>MSEFNITETYLRFLEEDTEMTMPIAAIEALVTLLRIKTPETAAEMINTIKSSTEELIKSIPNSVSLRAGCDIFMRFVLRNLHLYGDWENCKQHLIENGQLFVSRAKKSRNKIAEIGVDFIADDDIILVHGYSRAVFSLLNHAANKFIRFRCVVTESRPSKQGNQLYTLLEQKGIPVTLIVDSAVGAVIDKVDKVFVGAEGVAESGGIINLVGTYSVGVLAHNARKPFYVVTESHKFVRMFPLSSDDLPMAGPPLDFTRRTDDLEDALRGPTIDYTAQEYITALITDLGVLTPSAVSEELIKMWYD[2x];>MSESEAKSRSATPPSKAKQATPTTTAAANGEKKLTNKELKELKKQEKAAKRAAMKQANGISIEQQQQQAQMKKEKKQLQREQQQKREQKQKNANKKKQNERNVKKSTLFGHLETTEERRATILALTSAVSSPKTSRITAAGLMVPVVASALSGSNVLTASSLMPVGPNASSTVSASAPASTTTTLPASSAALSAGTSSASTNTPTAIQQEIASSNASDVAKTLASISLEAGEFNVIPGISSVIPTVLEQSFDNSSLISSVKELLLNKDLIHPSILLLTSHLAHYKIVGSIPRCIAMLEVFQIVIKDYQTPKGTTLSRNLTSYLSHQIDLLKKARPLSVTMGNAIRWLKQEISLIDPSTPDKAAKKDLCEKIGQFAKEKIELADQLIIDNASTQIEESTTIVTYGSSKVLTELLLHNAISLKKNIKVIVVDSRPLFEGRKMAETLRNAGVNVMYALITSLDTIFNMDVDYVFLGAHSILSNGFLYSRAGTAMLAMSAKRRNIPVLVCCESLKFSQRVQLDSVTFNELADPNDLVNIDYENPVERRGNKGALLNQFIKERKFEKKKLAMENKPKGNKIGGKKGSEGESKDASNEEDSNSKNILDGWQELPSLNIVNILYDLTPPEYIKKVITEFGALPPSSVPVILREYKGSA[2x];>[2x]MSSQAFTSVHPNAATSDVNVTIDTFVAKLKRRQVQGSYAIALETLQLLMRFISAARWNHVNDLIEQIRDLGNSLEKAHPTAFSCGNVIRRILAVLRDEVEEDTMSTTVTSTSVAEPLISSMFNLLQKPEQPHQNRKNSSGSSSMKTKTDYRQVAIQGIKDLIDEIKNIDEGIQQIAIDLIHDHEILLTPTPDSKTVLKFLITARERSNRTFTVLVTEGFPNNTKNAHEFAKKLAQHNIETLVVPDSAVFALMSRVGKVIIGTKAVFVNGGTISSNSGVSSVCECAREFRTPVFAVAGLYKLSPLYPFDVEKFVEFGGSQRILPRMDPRKRLDTVNQITDYVPPENIDIYITNVGGFNPSFIYRIAWDNYKQIDVHLDKNKA;>MAGKKGQKKSGLGNHGKNSDMDVEDRLQAVVLTDSYETRFMPLTAVKPRCLLPLANVPLIEYTLEFLAKAGVHEVFLICSSHANQINDYIENSKWNLPWSPFKITTIMSPEARCTGDVMRDLDNRGIITGDFILVSGDVLTNIDFSKMLEFHKKMHLQDKDHISTMCLSKASTYPKTRTIEPAAFVLDKSTSRCIYYQDLPLPSSREKTSIQIDPELLDNVDEFVIRNDLIDCRIDICTSHVPLIFQENFDYQSLRTDFVKGVISSDILGKHIYAYLTDEYAVRVESWQTYDTISQDFLGRWCYPLVLDSNIQDDQTYSYESRHIYKEKDVVLAQSCKIGKCTAIGSGTKIGEGTKIENSVIGRNCQIGENIRIKNSFIWDDCIIGNNSIIDHSLIASNATLGSNVRLNDGCIIGFNVKIDDNMDLDRNTKISASPLKNAGSRMYDNESNEQFDQDLDDQTLAVSIVGDKGVGYIYESEVSDDEDSSTEACKEINTLSNQLDELYLSDDSISSATKKTKKRRTMSVNSIYTDREEIDSEFEDEDFEKEGIATVERAMENNHDLDTALLELNTLRMSMNVTYHEVRIATITALLRRVYHFIATQTLGPKDAVVKVFNQWGLLFKRQAFDEEEYIDLMNIIMEKIVEQSFDKPDLILFSALVSLYDNDIIEEDVIYKWWDNVSTDPRYDEVKKLTVKWVEWLQNADEESSSEEE[2x];>[2x]MSIQAFVFCGKGSNLAPFTQPDFPFQTQNKDSTAATSGDKLNELVNSALDSTVINEFMQHSTRLPKALLPIGNRPMIEYVLDWCDQADFKEISVVAPVDEIELIESGLTSFLSLRKQQFELIYKALSNSNHSHHLQDPKKINFIPSKANSTGESLQKELLPRINGDFVILPCDFVTDIPPQVLVDQFRNRDDNNLAMTIYYKNSLDSSIDKKQQQKQKQQQFFTVYSENEDSERQPILLDVYSQRDVTKTKYLQIRSHLLWNYPNLTVSTKLLNSFIYFCSFELCQLLKLGPQSMSRQASFKDPFTGNQQQQNPPTTDDDEDRNHDDDDDYKPSATSIQPTYFKKKNDLILDPINCNKSLSKVFRDLSRRSWQHSKPREPIGIFILPNETLFIRANNLNAYMDANRFVLKIKSQTMFTKNIQIQSAAIGADAIVDPKCQISAHSNVKMSVLGTQANIGSRCRVAGSLLFPGVHLGDEVILENCIIGPMAKIGSKCKLSNCYIEGHYVVEPKNNFKGETLANVYLDEDEEDELIYDDSVIAGESEIAEETDSDDRSDEDSDDSEYTDEYEYEDDGLFER;>MSTSHCRFYENKYPEIDDIVMVNVQQIAEMGAYVKLLEYDNIEGMILLSELSRRRIRSIQKLIRVGKNDVAVVLRVDKEKGYIDLSKRRVSSEDIIKCEEKYQKSKTVHSILRYCAEKFQIPLEELYKTIAWPLSRKFGHAYEAFKLSIIDETVWEGIEPPSKDVLDELKNYISKRLTPQAVKIRADVEVSCFSYEGIDAIKDALKSAEDMSTEQMQVKVKLVAAPLYVLTTQALDKQKGIEQLESAIEKITEVITKYGGVCNITMPPKAVTATEDAELQALLESKELDNRSDSEDDEDESDDE[2x];>[2x]MSSDLAAELGFDPALKKKKKTKKVIPDDFDAAVNGKENGSGDDLFAGLKKKKKKSKSVSADAEAEKEPTDDIAEALGELSLKKKKKKTKDSSVDAFEKELAKAGLDNVDAESKEGTPSANSSIQQEVGLPYSELLSRFFNILRTNNPELAGDRSGPKFRIPPPVCLRDGKKTIFSNIQDIAEKLHRSPEHLIQYLFAELGTSGSVDGQKRLVIKGKFQSKQMENVLRRYILEYVTCKTCKSINTELKREQSNRLFFMVCKSCGSTRSVSSIKTGFQATVGKRRRM;>[2x]MSDLQDQEPSIIINGNLEPVGEPDIVEETEVVAQETQETQDADKPKKKVAFTGLEEDGETEEEKRKREFEEGGGLPEQPLNPDFSKLNPLSAEIINRQATINIGTIGHVAHGKSTVVRAISGVQTVRFKDELERNITIKLGYANAKIYKCQEPTCPEPDCYRSFKSDKEISPKCQRPGCPGRYKLVRHVSFVDCPGHDILMSTMLSGAAVMDAALLLIAGNESCPQPQTSEHLAAIEIMKLKHVIILQNKVDLMREESALEHQKSILKFIRGTIADGAPIVPISAQLKYNIDAVNEFIVKTIPVPPRDFMISPRLIVIRSFDVNKPGAEIEDLKGGVAGGSILNGVFKLGDEIEIRPGIVTKDDKGKIQCKPIFSNIVSLFAEQNDLKFAVPGGLIGVGTKVDPTLCRADRLVGQVVGAKGHLPNIYTDIEINYFLLRRLLGVKTDGQKQAKVRKLEPNEVLMVNIGSTATGARVVAVKADMARLQLTSPACTEINEKIALSRRIEKHWRLIGWATIKKGTTLEPIA

Eukaryotic protein synthesis typically begins with a specialised initiator methionyl transfer RNA (Met-tRNAi) that is delivered to ribosomes by the translation factor eIF2 as part of a larger preinitiation complex (PIC) with multiple other translation initiation factors. Only by re-engaging with GTP can eIF2 participate in further rounds of Met-tRNAi binding and protein synthesis initiation. This requires the action of eIF2B. eIF2B first removes eIF57 and then acts as a guanine nucleotide exchange factor (GEF) to activate eIF2 and facilitate Met-tRNAi interaction and rebinding of eIF53. Structural studies of eIF2B have shown that it is a decamer or a dimer of pentamers. eIF2B has a central hexameric core comprising an eIF2Bα homodimer and (βδ)2 heterotetramer that is linked to a pair of γε heterodimeric arms. Here we have used single-particle electron cryomicroscopy (cryoEM) to resolve the structures of eIF2αP/eIF2B and eIF2/eIF2B complexes from Saccharomyces cerevisiae to an average resolution of 3.9 and 4.6 Å, respectively.

The yeast strains used are deleted for the sole eIF2α kinase Gcn2; hence, eIF2 is purified uniformly dephosphorylated at the ISR regulatory site. The 3D map generated for this eIF2/eIF2B complex is remarkably similar to the eIF2αP/eIF2B complex, with two eIF2 molecules bound one at each side of the eIF2B decamer. Therefore, to build the atomic model for this complex, our eIF2αP/eIF2B core model (eIF2B with eIF2α domains 1 and 2) provided the initial eIF2α/eIF2B atomic coordinates. Hence, the eIF2B subunit structural models are highly similar, with only very minor rearrangements. When the Ser52 loop of eIF2α is examined closely, one clear local difference is loss of the density associated with the S52 phosphate. Specifically, R53 is reoriented in the unphosphorylated complex. In addition, there are minor movements associated with R55 and R64, the latter moves away from S52. The density around R54 is weaker in eIF2/eIF2B than in the eIF2αP/eIF2B complex structure, suggesting that it may adopt more than one position. Overall, the weaker density in the S52 phospho-loop of the eIF2/eIF2B complex prevents us defining precisely the positions of the side chains. This likely points to enhanced flexibility of this region of eIF2α in the absence of the phosphate group.(6S)-6-[5-(3,5-dimethyl-1,2-oxazol-4-yl)-1-[(3R)-1-methylsulfonylpyrrolidin-3-yl]benzimidazol-2-yl]-1-(3-fluoranyl-4-methoxy-phenyl)piperidin-2-one 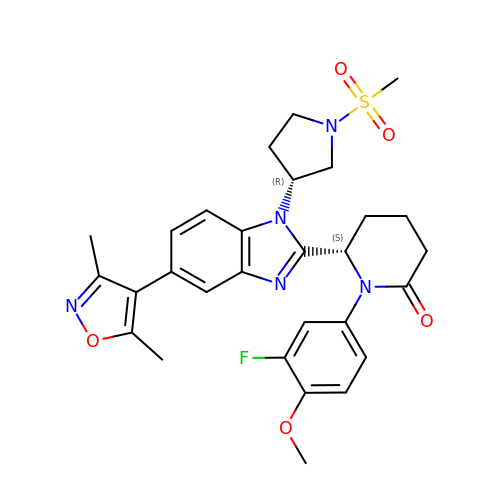| C29 H32 F N5 O5 S | IXWWSEVQKVTANB-BWKNWUBXSA-N>[2x]PFITVGQENSTSIDLYYEDHGAGQPVVLIHGFPLSGHSWERQSAALLDAGYRVITYDRRGFGQSSQPTTGYDYDTFAADLNTVLETLDLQDAVLVGFSMGTGEVARYVSSYGTARIAKVAFLASLEPFLLKTDDNPDGAAPKEFFDGIVAAVKADRY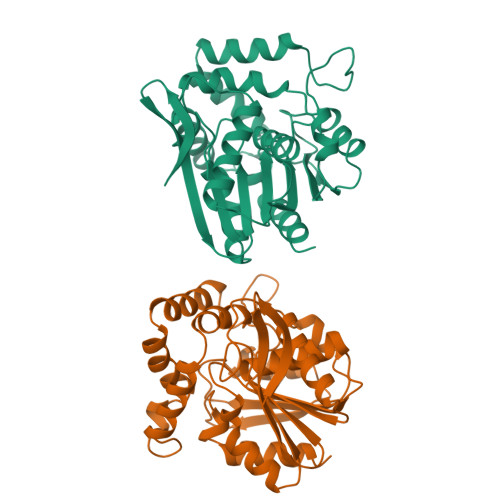AFYTGFFNDFYNLDENLGTRISEEAVRNSWNTAASGGFFAAAAAPTTWYTDFRADIPRIDVPALILHGTGDRTLPIENTARVFHKALPSAEYVEVEGAPHGLLWTHAEEVNTALLAFLAK>MATQTSKNPESVHDFTVKDAKENDV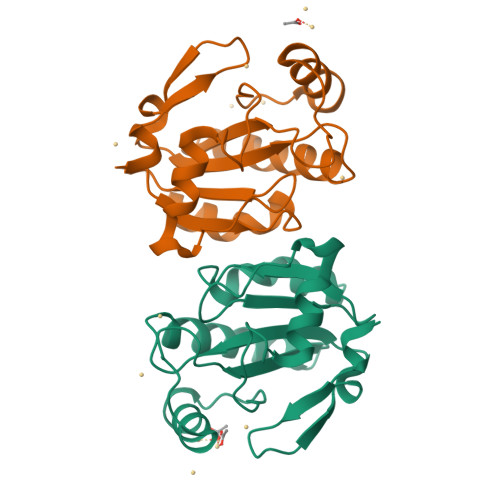DLSIFKGKVLLIVNVASKCGMTNSNYAEMNQLYEKYKDQGLEILAFPCNQFGEEEPGTNDQITDFVCTRFKSEFPIFDKIDVNGENASPLYRFLKLGKWGIFGDDIQWNFAKFLVNKDGQVVDRYYPTTSPLSLERDIKQLLEIS[4x]> ADKELKFLVVDDFSTMRRIVRNLLKELGFNNVEEAEDGVDALNKLQAGGFGFIISDWNMPNMDGLELLKTIRA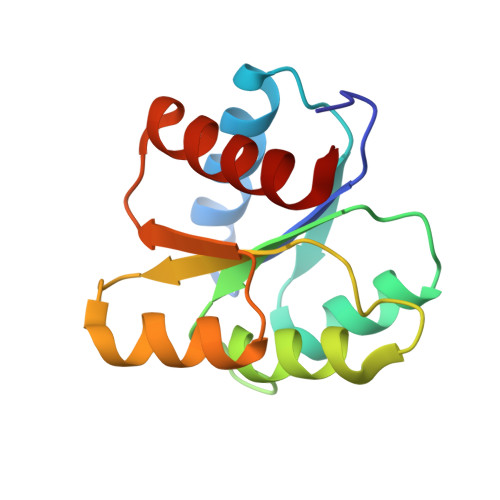DSAMSALPVLMVTAEAKKENIIAAAQAGASGYVVKPFTAATLEEKLNKIFEKLGM> PECFTANGADYRGTQNWTALQGGKPCLFWNETFQHPYNTLKYP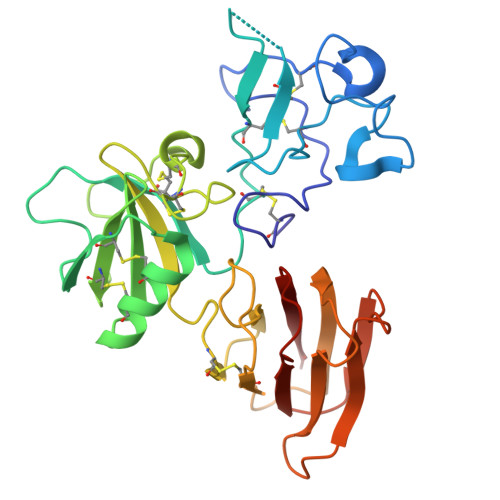NGEGGLGEHNYCRNPDGDVSPWCYVAEHEDGVYWKYCEIPACQMPGNLGCYKDHGNPPPLTGTSKTSNKLTIQTCISFCRSQRFKFAGMESGYACFCGNNPDYWKYGEAASTECNSVCFGDHTQPCGGDGRIILFDTLVGACGGNYSAMSSVVYSPDFPDTYATGRVCYWTIRVPGASHIHFSFPLFDIRDSADMVELLDGYTHRVLARFHGRSRPPLSFNVSLDFVILYFFSDRINQAQGFAVLYQAVK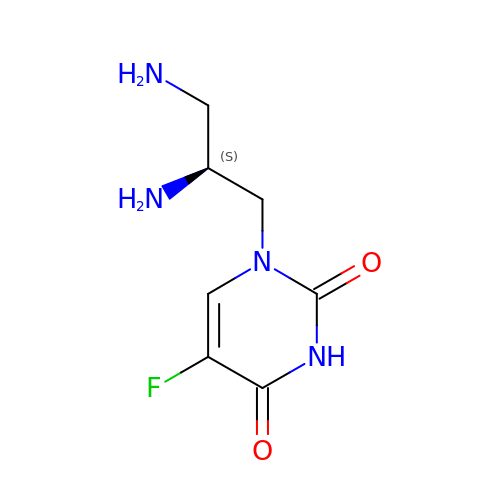1-[(2S)-2,3-diaminopropyl]-5-fluoropyrimidine-2,4(1H,3H)-dione | C7 H11 F N4 O2 | ZBKWVMMCABYTAU-BYPYZUCNSA-N>DSYYQRSDWTADEEQILLGPFDYLESLPGKNMRSQLIQSFNTWLKVPTESLDVIIKVISMLHTATLLIDDIQDQSILRRG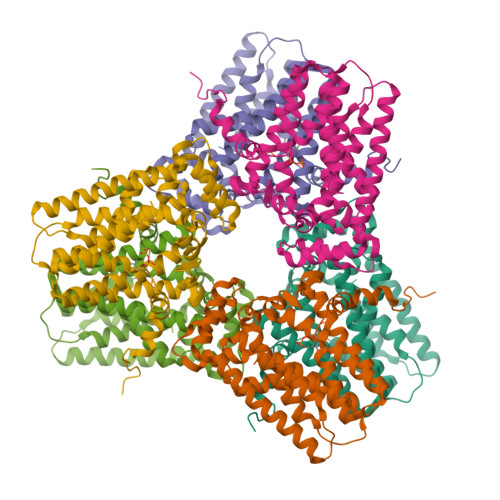QPVAHSIFGTAQAMNSGNYVYFLALREVQKLQNPKAISIYVDSLIDLHRGQGMELFWRDSLMCPTEEQYLDMVANKTGGLFCLAIQLMQAEATIQVDFIPLVRLLGIIFQICDDYLNLKSTAYTDNKGLCEDLTEGKFSFPIIHSIRSNPGNRQLINILKQKPREDDIKRYALSYMESTNSFEYTRGVVRKLKTEAIDTIQGLEKHGLEENIGIRKILARMSLEL[2x]> MAFAPIPRITWEHREVHLVQFHEPDIYNYSAL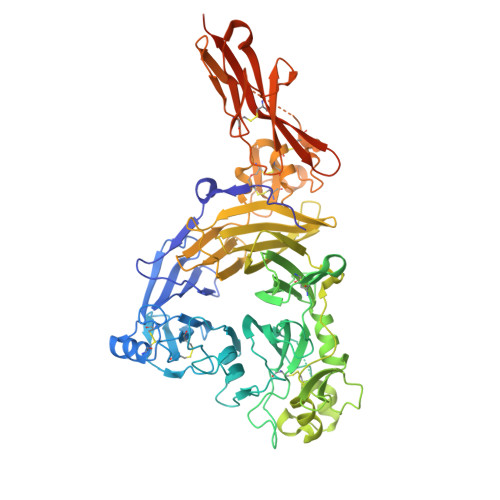LLSEDKDTLYIGAREAVFAVNALNISEKQHEVYWKVSEDKKAKCAEKGKSKQTECLNYIRVLQPLSATSLYVCGTNAFQPACDHLNLTSFKFLGKNEDGKGRCPFDPAHSYTSVMVDGELYSGTSYNFLGSEPIISRNSSHSPLRTEYAIPWLNEPSFVFADVIRKSPDSPDGEDDRVYFFFTEVSVEYEFVFRVLIPRIARVCKGDQGGLRTLQKKWTSFLKARLICSRPDSGLVFNVLRDVFVLRSPGLKVPVFYALFTPQLNNVGLSAVCAYNLSTAEEVFSHGKYMQSTTVEQSHTKWVRYNGPVPKPRPGACIDSEARAANYTSSLNLPDKTLQFVKDHPLMDDSVTPIDNRPRLIKKDVNYTQIVVDRTQALDGTVYDVMFVSTDRGALHKAISLEHAVHIIEETQLFQDFEPVQTLLLSSKKGNRFVYAGSNSGVVQAPLAFCGKHGTCEDCVLARDPYCAWSPPTATCVALHQTESPSRGLIQEMSGDASVCPDKSKGSYRQHFFKHGGTAELKCSQKSNLARVFWKFQNGVLKAESPKYGLMGRKNLLIFNLSEGDSGVYQCLSEERVKNKTVFQVVAKHVLEVKVVPKPVVAPTLSVVQTEGSRIATKVLVASTKHHHHHH>[4x]MNLEKINELTAQDMAGVNAAILEQLNSDVQLINQLGYYIVSGGGKRIRPMIAVLAARAVGYEGNAHVTIAALIEFIHTATLLHDDVVDESDMRRGKATANAAFGNAASVLVGDFIYTRAFQMMTSLGSLKVLEVMSEAVNVIA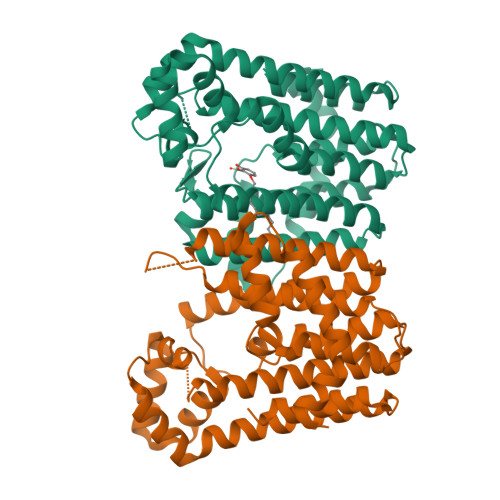EGEVLQLMNVNDPDITEENYMRVIYSKTARLFEAAAQCSGILAGCTPEEEKGLQDYGRYLGTAFQLIDDLLDYNADGEQLGKNVGDDLNEGKPTLPLLHAMHHGTPEQAQMIRTAIEQGNGRHLLEPVLEAMNACGSLEWTRQRAEEEADKAIAALQVLPDTPWREALIGLAHIAVQRDR> GSAKDPGQIRGLEMASKNSQDGISLIQTAEGALTETHAILQRMRELTVQAGNTGTQ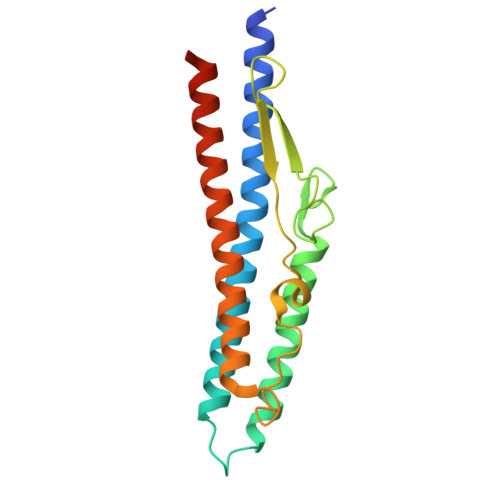QAEDLGAIKDEMDALIEEIDGISNRTEFNGKKLLDGTNSTDGFTFQIGANAGQQLNVKIDSMSSTALGVNALDVTDFAATAFDDQLKSIDTAINTVSTQRAKLGAVQNRLEHTINNLGASGENLTAA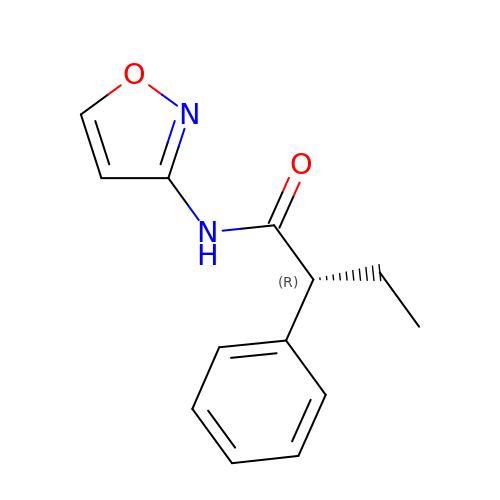(2R)-N-(1,2-oxazol-3-yl)-2-phenylbutanamide | C13 H14 N2 O2 | SZRQFFYFLMVKTJ-LLVKDONJSA-N Cyclic nucleotide phosphodiesterases (PDEs) hydrolyze the second messengers cAMP and cGMP, and play crucial roles in many physiological processes. PDE molecules contain an N-terminal regulatory domain and a conserved catalytic domain at the C-terminus. To understand the roles of the invariant glutamine, we mutated Gln453 of PDE9A2 to glutamic acid (PDE9Q453E) and its stabilizing residue Glu406 to alanine, and measured the kinetic parameters of the mutants. In addition, we performed molecular dynamics (MD) simulations on the mutants and determined the crystal structures of PDE9Q453E in complex with the inhibitors 3-isobutyl-1-methylxanthine (IBMX) and (S)-BAY73-6691.

In the Q453E mutant structure, the side chain of Glu453 rotated about 15°. This movement made a distance of 3.8 Å from OE2 of Glu453 to O4 of (S)-BAY73-6691, and 3.2 Å to OE1 of Glu406. The 3.2 Å distance between two electron-rich oxygen atoms may cause energetically unfavored repulsion. A possible explanation may be that Glu406 is protonated, as discussed in the section on MD simulations. In the PDE9Q453E-(S)-BAY73-6691 structure, the conformation and position of (S)-BAY73-6691 to chain A was clearly defined by the electron density maps of (2Fo - Fc) and (Fo - Fc). However, the electron density in chain B had the quality only to reveal the binding location but not the accurate conformation of the inhibitor. In chain A, the pyrazolo-pyrimidine ring of (S)-BAY73-6691 stacked against the phenyl ring of Phe456 and its N5 atom formed a hydrogen bond with OE1 of Glu453. In chain B, (S)-BAY73-6691 formed no hydrogen bond with Glu453, but with Tyr424, although its pyrazolo-pyrimidine ring remained stacked against Phe456. The IC50 value of (S)-BAY73-6691 for the PDE9Q453E mutant was >160 µM, which is >1800 fold to IC50 of 86 nM for the wild type enzyme. However, since the selective PDE9 inhibitor (S)-BAY73-6691 fits tightly to the binding pocket, the Q453E mutation would cause a net loss of the hydrogen bond and thus impact on the binding affinity.

>[2x]MGSGSSSYRPKAIYLDIDGRIQKVIFSKYCNSSDIMDLFCIATGLPRNTTISLLTTDDAMVSIDPTMPANSERTPYKVRPVAIKQLSEREELIQSVLAQVAEQFSRAFKINELKAEVANHLAVLEKRVELEGLKVVEIEKCKSDIKKMREELAARSSRTNCPCKYSFLDNHKKLTPRRDVPTYPKYLLSPETIEALRKPTFDVWLWEPNEMLSCLEHMYHDLGLVRDFSINPVTLRRWLFCVHDNYRNNPFHNFRHCFCVAQMMYSMVWLCSLQEKFSQTDILILMTAAICHDLDHPGYNNTYQINARTELAVRYNDISPLENHHCAVAFQILAEPECNIFSNIPPDGFKQIRQGMITLILATDMARHAEIMDSFKEKMENFDYSNEEHMTLLKMILIKCCDISNEVRPMEVAEPWVDCLLEEYFMQSDREKSEGLPVAPFMDRDKVTKATAEIGFIKFVLIPMFETVTKLFPMVEEIMLQPLWESRDRYEELKRIDDAMKELQKKTDSLTSGATEKSRERSRDVKNSEGDCA Bacillus cereus (Bc) encodes three FNR paralogs, two of which have assigned distinct biological functions in bacillithiol disulfide reduction and flavodoxin (Fld) reduction. In this study, we have assigned a function to FNR1, in which the His residue is replaced by a conserved Val, in the reduction of the heme-degrading monooxygenase IsdG, ultimately facilitating the release of iron in an important iron acquisition pathway. The Bc IsdG structure was solved, and IsdG-FNR1 interactions were proposed through protein–protein docking. Mutational studies and bioinformatics analyses confirmed the importance of the conserved FAD-stacking residues on the respective reaction rates, proposing a division of FNRs into four functionally unique sequence similarity clusters likely related to the nature of this residue.

The IsdG monomers consist of Fd-like α/β-sandwich folds forming a β-barrel at the dimeric interface containing the conserved Asn-Trp-His triad required for the catalytic activity in the heme binding pockets. Bc IsdG was crystallized in its apo-form and reconstituted with hemin, the latter yielding red-brownish crystals. The electron density for the heme groups of IsdGheme was, however, relatively poor, and only 50% occupancy could be modeled, with apparent density for the iron ions but limited for the rest of the porphyrin. In addition to low occupancy, the heme groups might be bound with different orientations and degrees of ruffling. However, after the addition of FNR1 (after 950 s), the breakdown of heme is detected in the enzymatic reaction under aerobic conditions, confirming the importance of FNR1 for the degradation of heme in Bc IsdG and the resulting release of iron. Moreover, in the FNR1-catalyzed reaction, the decrease of the Soret peak detected at 427 nm demonstrates the breakdown of the heme-bound Fe(II) state, which is not observed for the non-enzymatic NADPH-driven reaction, where, instead, a build-up of heme-bound Fe(II) occurs.

>[2x]MIIVTNTAKITKGNGHKLIERFNKVGKVETMPGFLGLEVLLTQNTVDYDEVTISTRWNAKEDFQGWTKSAAFKDAHSHQGGMPEYILDNKIAYYDVKVVRMPMAAAQ> MELQQNFTDNNSIKYTCILILIAFAFSVLCRLYWVAWASEFYEFFFNDQLMITTNDGYAFAEGARDMIAGFHQPNDLSYFGSSLSTLTYWLYSILPFSFESIILYMSTFFASLIVVPIILIAREYKLTTYGFIAALLGSIANSYYNRTMSGYYDTDMLVLVLPMLILLTFIRLTINKDIFTLLLSPIFIMIYLWWYPSSYSLNFAMIGLFGLYTLVFHRKEKIFYLAIALMIIALSMLAWQYKLALIVLLFAIFAFKEEKINFYMIWALIFISISILHLSGGLDPVLYQLKFYVFKASDVQNLKDAAFMYFNVNETIMEVNTIDPEVFMQRISSSVLVFILSFIGFILLCKDHKSMLLALPMLALGFMALRAGLRFTIYAVPVMALGFGYFLYAFFNFLEKKQIKLSLRNKNILLILIAFFSISPALMHIYYYKSSTVFTSYEASILNDLKNKAQREDYVVAWWDYGYPIRYYSDVKTLIDGGKHLGKDNFFSSFVLSKEQ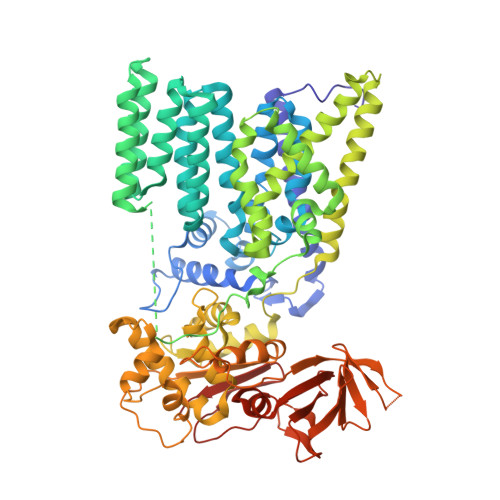IPAANMARLSVEYTEKSFKENYPDVLKAMVKDYNQTSAKDFLESLNDKNFKFDTNKTRDVYIYMPYRMLRIMPVVAQFANTNPDNGEQEKSLFFSQANAIAQDKTTGSVMLDNGVEIINDFRALKVEGASIPLKAFVDIESITNGKFYYNEIDSKAQIYLLFLREYKSFVILDESLYNSAYIQMFLLNQYDQDLFEQVTNDTRAKIYRLKREFHHHHHHHHHH>SDFVVIKAVEDGVNVIGLTRG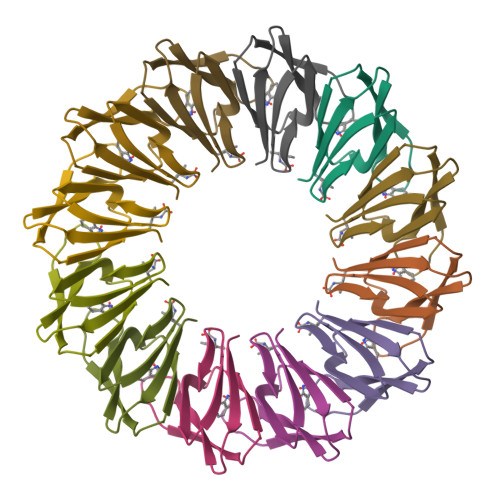TDTKFHHSEKLDKGEVIIAQFTEHTSAIKVRGEALIQTAYGEMK[6x]>QLRYSVVEESEPGTLVGNVAQDLGLKGTDLLSRRLRLGSEENGRYFSLSLVSGALAVSQKIDRESLCGASTSCLLPVQVVTEHPLELTRVEVEILDLNDNSPSFATPDREMRISESAAPGARFPLDSAQDPDVGTNTVSFYTLSPNSHFSLHV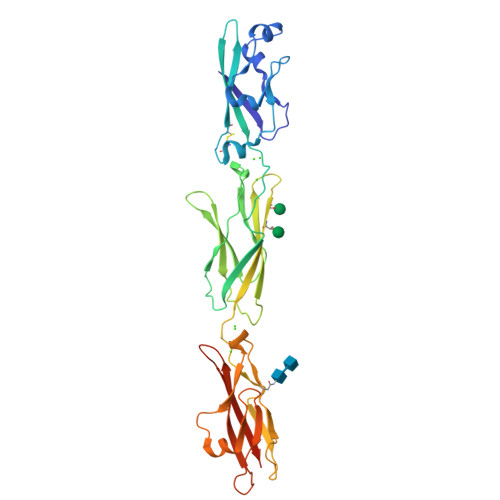KTLKDGKLFPELVLEQQLDRETQARHQLVLTAVDGGTPARSGTSLISVIVLDVNDNAPTFQSSVLRVGLPENTPPGTLLLRLNATDPDEGTNGQLDYSFGDHTSETVKNLFGLDPSSGAIHVLGPVDFEESNFYEIHARARDQGQPAMEGHCVIQVDVGDANDHHHHHHHH[2x]>SNAMLEIVLASQNSSKLAEMQELLRDLEIKFIPQTEFSVPDIEETGSTFVENAIIKARHAAKQTGLPALADDSGLTIAALNSAPGVFSSRYAGKNATDAERIQKVLEALEAADDSDRSASFHCVIALMENE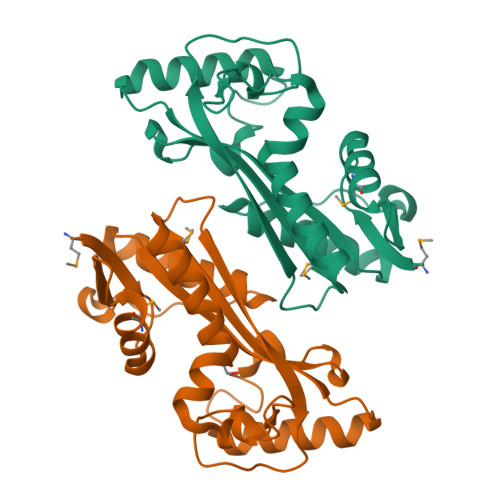NDPAPLICHGVWEGEIAREPRGKNGFGYDPIFYVPSHQRTAAELDPQEKNAISHRGQALEQLSTVLTEAFLV[4x]>[4x]ADTIVAVELDTYPNTDIGDPSYPH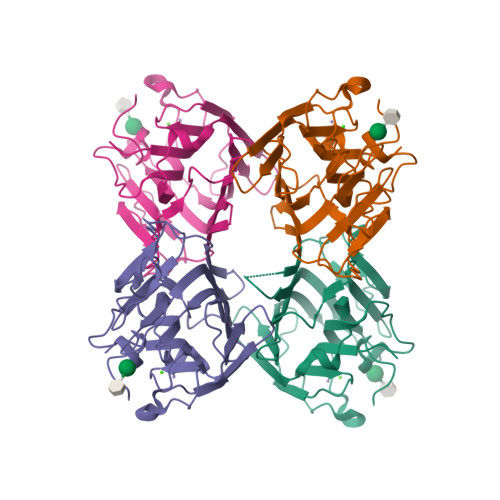IGIDIKSVRSKKTAKWNMQNGKVGTAHIIYNSVGKRLSAVVSYPNGDSATVSYDVDLDNVLPEWVRVGLSASTGLYKETNTILSWSFTSKLKSNSTHETNALHFVFNQFSKDQKDLILQGDATTGTDGNLELTRVSSNGSPQGSSVGRALFYAPVHIWESSAVVASFDATFTFLIKSSDSHPADGIAFFISNIDSSIPSGSTGRLLGLFPDAN>GGVLNMIEITYIDASKNERTVTFESYEDFERSQQACLIGVADYYPVQKLTYKGHNLDYHGTYGDIFFYLMKQ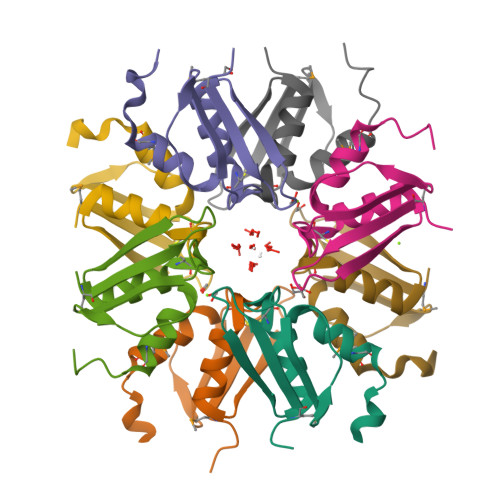DLSQYN[8x]> ADAAAGAQVFAANCAACHAGGNNAVMPTKTLKADALKTYLAGYKDGSKSLEE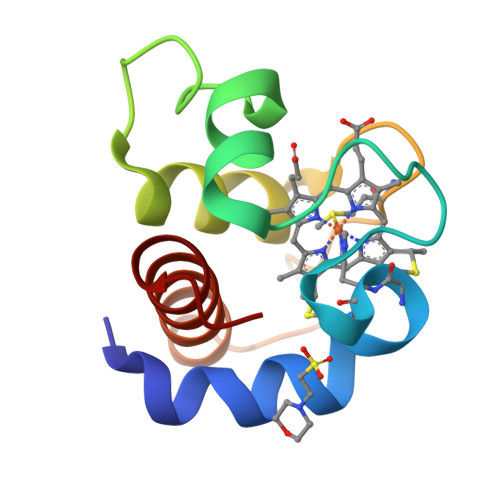AVAYVVTNGQGAMPAFGGRLSDADIANVAAYIADQAENNKW> MPTRANVLDKRKVGNLSGGVNYFAADPRIKNVEALDKKLLAYLDKHGEDSTIGMRAIITIL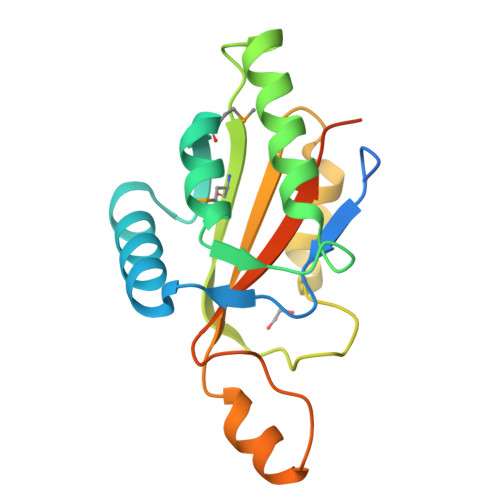NAFTVDPNDLDLATFKAALLDFERNQPHLTARMVLRTNRKVNQGTGALLSPTDQALSRAEVAHPLLILYRIEGVNDAAAQRGEPTWSSDPIWVPNIKLPGQRQFWCVDGGHHHHHHG>[2x]MGNIRYSVPEETDKGSFVGSIAKDLGLETRELMERGIRIVSRGRSQLFSLNPRSGSLVTAGRIDREELCAQSTPCVVSFNILMEDEMKLLPIEVEIIDINDNTPQFQLEELELKMSEITTPGTRIPLPLGQDLDVGINSLQSYQLSANPHFSLDVQQGPEGPQQPEMVLQRPLDREKDAVHYLVLTASDGGSPIHSGT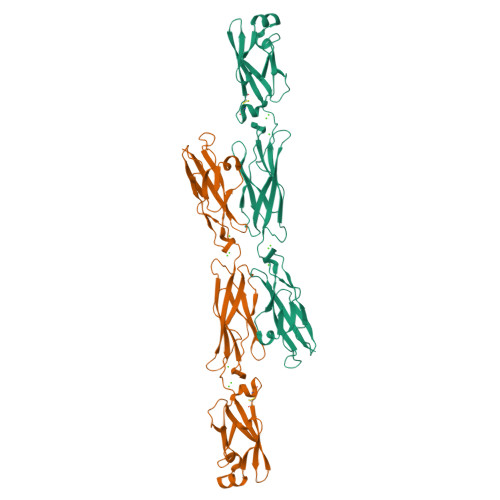LQIHVQVVDVNDNPPAFTKAEYHVSVPENVPLGTRLLKVNATDPDEGANGRVTYSFHKVDHSVVRKFQLDAYTGELSNKEPLDFEEYKVYPMEIQAQDGAGLMARAKVLVTVLDHHHHHH2,2-difluoroethyl (3S)-3-{[2'-amino-5-fluoro-2-(morpholin-4-yl)[4,5'-bipyrimidin]-6-yl]amino}-3-(hydroxymethyl)pyrrolidine-1-carboxylate 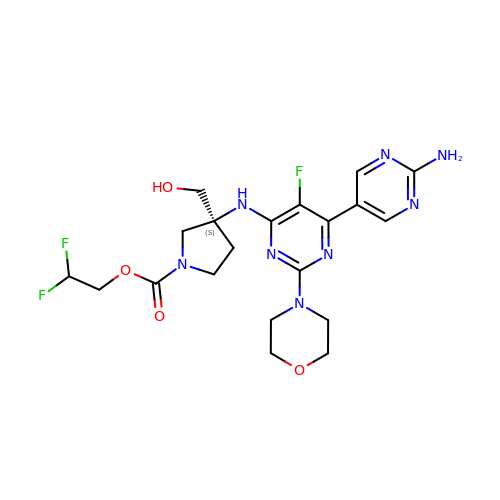| C20 H25 F3 N8 O4 | RTOREZYNLPQUKM-FQEVSTJZSA-N> MHHHHHHAVRASEISRVYEAYPEKKATLYFLVLGFLALIVGSLFGPFQALNYGNVDAYPLLKRLLPFVQSYYQGLTLHGVLNAIVFTQLFAQAIMVYLPARELNMRPNMGLMWLSWWMAFIGLVVAALPLLANEATVLFTFYPPLKGHWAFYLGASVFVLSTWVSIYIVLDLWRRWKAANPGKVTPLVTYMAVVFWLMWFLASLGLVLEAVLFLLPWSFGLVEGVDPLVARTLFWWTGHPIVYFWLLPAYAIIYTILPKQAGGKLVSDPMARLAFLLFLLLSTPVGFHHQFADPGIDPTWKMIHSVLTLFVAVPSLMTAFTVAASLEFAGRLRGGRGLFGWIRALPWDNPAFVAPVLGLLGFIPGGAGGIVNASFTLDYVVHNTAWVPGHFHLQVASLVTLTAMGSLYWLLPNLTGKPISDAQRRLGLAVVWLWFLGMMIMAVGLHWAGLLNVPRRAYIAQVPDAYPHAAVPMVFNVLAGIVLLVALLLFIYGLFSVLLSRE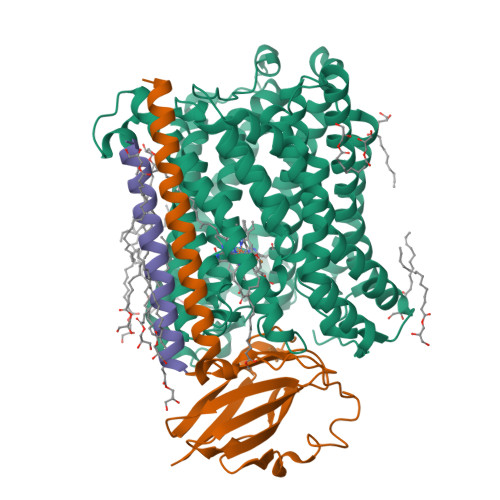RKPELAEAPLPFAEVISGPEDRRLVLAMDRIGFWFAVAAILVVLAYGPTLVQLFGHLNPVPGWRLW;> MVDEHKAHKAILAYEKGWLAFSLAMLFVFIALIAYTLATHTAGVIPAGKLERVDPTTVRQEGPWADPAQAVVQTGPNQYTVYVLAFAFGYQPNPIEVPQGAEIVFKITSPDVIHGFHVEGTNINVEVLPGEVSTVRYTFKRPGEYRIICNQYCGLGHQNMFGTIVVKE;> MEEKPKGALAVILVLTLTILVFWLGVYAVFFARG> GFPTELKPGTNQF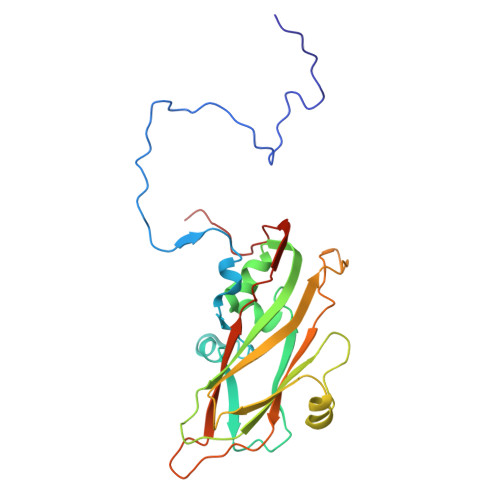LTTDDGVSAPILPNFYPTPCIHIPGEVRNLLELCQVETILEVNNVPTNATSLMERLRFPVSAQAGKGELCAVFRADPGRSGPWQSTLLGQLCGYYTQWSGSLEVTFMFTGSFMATGKMLIAYTPPGGPLPKDRATAMLGTHVIWDFGLQSSVTLVIPWISNTHYRAHARDGVFDYYTTGLVSIWYQTNYVVPIGAPNTAYIIALAAAQKNFTMKLCKDASDILQTGTIQ Type I CRISPR-Cas systems employ multi-subunit effector Cascade and helicase-nuclease Cas3 to target and degrade foreign nucleic acids, representing the most abundant RNA-guided adaptive immune systems in prokaryotes. Here, we present two cryo-EM structures of the Synechocystis sp. PCC 6714 (Syn) type I-B Cascade, revealing the molecular mechanisms that underlie RNA-directed Cascade assembly, target DNA recognition, and local conformational changes of the effector complex upon R-loop formation. The stoichiometry of SynCascade was Cas8b1-Cas7b7-Cas5b1-Cas6b1-Cas11b3. Taken together, these results suggest that both the “GNS” loop of Cas5b and the “GVP” loop of Cas8b are responsible for AYG-PAM recognition in Syn type I-B Cascade.

To elucidate the detailed mechanism of how the Syn type I-B Cascade recognizes target DNA, we incubated a 59-bp dsDNA target containing an ATG-PAM with SynCascade in a 1:3 molar ratio at 25 °C for 1 h, the unbound dsDNA was then removed by SEC purification. The final 3D reconstruction reached an overall resolution higher than 3.6 Å, which was sufficient to identify the direction of the main chain and the clear side chains. The target strand (TS) is embedded within the complex and hybridized with the crRNA, representing the full R-loop formed state. However, the non-target strand (NTS) was not fully visible, particularly the bulge for Cas3 recruitment. In our full R-loop state structure, we modeled 6 bp of PAM-proximal dsDNA and 19 nt of NTS ssDNA. Out of these, 9 nt of NTS ssDNA were directly located downstream of PAM, while the other 10 nt constituted the PAM-distal region stabilized by the small subunits were modeled using “A”. Positively charged residues (R88, R159, K244, R245 and R282) within the Cas8b NTD made sequence-independent contacts with the negatively charged NTS backbone. In addition to electrostatic contacts, we identified aromatic residues (Y119 and F281) of Cas8b NTD that participated in the stacking interactions with NTS bases, which stabilizing the single-stranded region of the NTS seed. Comparative analysis of the overall structure of Cas8b in the two different states showed that its CTD extended in the full R-loop structure, with an RMSD of 6.7 Å. Comparison of the “belly” in the two structures reveals a pivoting motion of the extended Cas8b CTD, accompanied by a correlated motion and rotation of the three Cas11b subunits reflected by an RMSD of 3.15 Å.

> MAQLALALDTVTRYLRLKAPFAAFRPFQSGSFRSTTPVPSFSAVYGLLLNLAGIEQRQEVEGKVTLIKPKAELPKLAIAIGQVKPSSTSLINQQLHNYPVGNSGKEFASRTFGSKYWIAPVRREVLVNLDLIIGLQSPVEFWQKLDQGLKGETVINRYGLPFAGDNNFLFDEIYPIEKPDLASWYCPLEPDTRPNQGACRLTLWIDRENNTQTTIKVFSPSDFRLEPPAKAWQQLPG;>[7x]MSNLNLFATILTYPAPASNYRGESEENRSVIQKILKDGQKYAIISPESMRNALREMLIELGQPNNRTRLHSEDQLAVEFKEYPNPDKFADDFLFGYMVAQTNDAKEMKKLNRPAKRDSIFRCNMAVAVNPYKYDTVFYQSPLNAGDSAWKNSTSSALLHREVTHTAFQYPFALAGKDCAAKPEWVKALLQAIAELNGVAGGHARAYYEFAPRSVVARLTPKLVAGYQTYGFDAEGNWLELSRLTATDSDNLDLPANEFWLGGELVRKMDQEQKAQLEAMGAHLYANPEKLFADLADSFLGV;> MPKTQAEILTLDFNLAELPSAQHRAGLAGLILMIRELKKWPWFKIRQKEKDVLLSIENLDQYGASIQLNLEGLIALFDLAYLSFTEERKSKSKIKDFKRVDEIEIEENGKNKIQKYYFYDVITPQGGFLAGWDKSDGQIWLRIWRDMFWSIIKGVPATRNPFNNRCGLNLNAGDSFSKDVESVWKSLQNAEKTTGQSGAFYLGAMAVNAENVSTDDLIKWQFLLHFWAFVAQVYCPYILDKDGKRNFNGYVIVIPDIANLEDFCDILPDVLSNRNSKAFGFRPQESVIDVPEQGALELLNLIKQRIAKKAGSGLLSDLIVGVEVIHAEKQGNSIKLHSVSYLQPNEESVDDYNAIKNSYYCPWFRRQLLLNLVNPKFDLASQSWLKRHPWYGFGDLLSRIPQRWLKENNSYFSHDARQLFTQKGDFDMTVATTKTREYAEIVYKIAQGFVLSKLSSKHDLQWSKCKGNPKLEREYNDKKEKVVNEAFLAIRSRTEKQAFIDYFVSTLYPHVRQDEFVDFAQKLFQDTDEIRSLTLLALSSQYPIKRQGETE;>MTVATTKTREYAEIVYKIAQGFVLSKLSSKHDLQWSKCKGNPKLEREYNDKKEKVVNEAFLAIRSRTEKQAFIDYFVSTLYPHVRQDEFVDFAQKLFQDTDEIRSLTLLALSSQYPIKRQGETE[3x]> TFISRFAPDQPRKGADILVEALERQGVETVFAYPGGASMEIHQALTRSSSIRNVLPRHEQGGVFAAEGYARSSGKPGICIATSGPGATNLVSGLADALLDSVPLVAITGQVTRRMIGTDAFQETPIVEVTRSITKHNYLVMDVEDIPRIIEEAFFLATSGRPGPVLVDVPKDIQQQLAIPNWEQAMRLPGYMSRMPKPPEDSHLEQIVRLISESKKPVLYVGGGCLNSSDELGRFVELTGIPVASTLMGLGSYPCDDELSLHMLGMHGTVYANYAVEHSDLLLAFGVRFDDRVTGKLEAFASRAKIVHIDIDSAEIGKNKTPHVSVCGDVKLALQGMNKVLENRAEELKLDFGVWRNELNVQKQKFPLSFKTFGEAIPPQYAIKVLDELTDGKAIISTGVGQHQMWAAQFYNYKKPRQWLSSGGLGAMGFGLPAAIGASVANPDAIVVDIDGDGSFIMNVQELATIRVENLPVKVLLLNNQHLGMVMQWEDRFYKANRAHTFLGDPAQEDEIFPNMLLFAAACGIPAARVTKKADLREAIQTMLDTPGPYLLDVICPHQEHVLPMIPSGGTFNDVITEGDGR

Acetohydroxyacid synthase (AHAS), also known as acetolactate synthase, is the first enzyme of the branched chain amino acid (BCAA) biosynthesis pathway, and is the target for more than 50 of these commercial herbicides. Since the introduction of these herbicides, 197 site-of-action resistance isolates have been identified. These sites are mainly focused on just eight amino acids 1 with all located in the substrate access channel or the catalytic pocket of AHAS. Here, we show that these mutations can have two effects (i) to reduce binding affinity of the herbicides and (ii) to abolish time-dependent accumulative inhibition, critical to the exceptional effectiveness of this class of herbicide.

Next, the crystal structure of the P197T mutant in complex with BS was determined. The P197T-BS complex is very similar to the structure of the WT AtAHAS-BS complex, with the polypeptides and the herbicides having near-identical conformations. In contrast to CE, BS interacts with T197. This feature and the fact that the interaction of the two heterocyclic rings is not affected by the P197 mutation may explain why the binding of BS is only weakly affected, with an increase in Ki of around three-fold compared to WT AtAHAS. Remarkably, the efficiency of accumulative inhibition by BS increases in the P197 mutant by approximatively two-fold. Altogether, these data suggest that the inhibition potency of BS is not affected by the P197 mutation. However, for BS accumulative inhibition was maintained for each mutant, and for the two P197 mutants the affinity of BS (Ki) remained high.> GLGDELEEVIVEKTKQTVASISSGPKHTQKVPILTANETGATMPVLPSDSIETRTTYMHFNGSETDVECFLGRAACVHVTEIQNKDATGIDNHREAKLFNDWKINLSSLVQLRKKLELFTYVRFDSEYTILATASQPDSANYSSNLVVQAMYVPPGAPNPKEWDDYTWQSASNPSVFF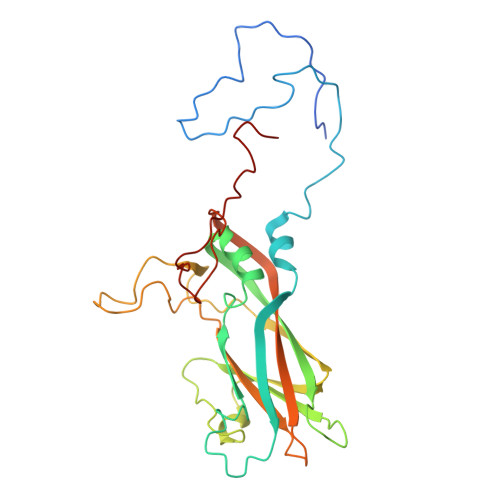KVGDTSRFSVPYVGLASAYNYFYDGYSHDDAETQYGITVLNHMGSMAFRIVNEHDEHKTLVKIRVYHRAKHVEAWIPRAPRALPYTSIGRTNYPKNTEPVIKKRKGDIKSY4-ethoxybenzoic acid | C9 H10 O3 | 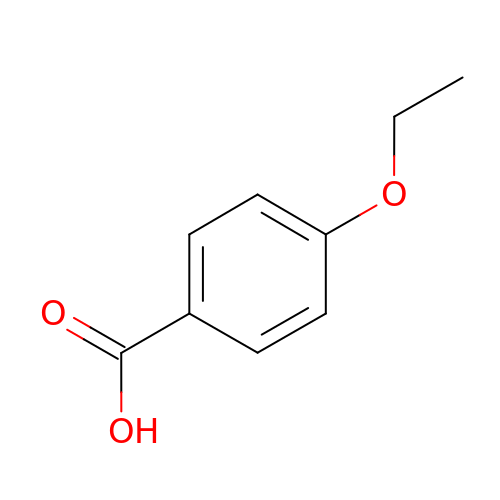SHSGDXCJYVZFTP-UHFFFAOYSA-N>[8x]MIDLNIMKVANYINGEFKEPSTGAFQVKTSPVDGSKIAEVPRSGREDAREAIDSAFEALKAWANIPAIRRAEYLYKMLEVFRQMKEDFMKILTVEGGGTYRKVWGEVVFTERLIQNAAELARHYQGRVLQSDSESTISVVFKRSKGVVGVITPWNYPLSISMKKIAHTLAVGNTVVYKPASDTPVTGWLIAQMVAKAGLPKGVFNLVIGPGPVVGEEIVTHKRVAHVTFTGESSTGREIAAKAAGTLKTVTLELGGSDPLIILDDVDVDYAARLAVFASLFHQGQICTSAKRIIVHKAVADKFIERYVHYVKMLRIDDPRKDEKVDLGPLINERQVALMKEFVDDAVSRGGRLLIGGRSWGNFFEPAIFVDVDRNFRIMREEVFGPVRPIVVVENDDQAVEVANDTDYGLSGAVLTNNVNRAFRIAEAVESGMFHINDVTFLEESHVPFGGIKASGVGREGGEWSFHETTYDRWVTVTLRTRRFPIPSALK

In the present work, we report the structural and functional characterization of the first thermostable archaeal dehydrogenase (AlDHPyr1147). The kinetic data showed that AlDHPyr1147 is strictly specific for NADP+ and is active with aliphatic aldehydes. According to gel filtration, AlDHPyr1147 is a tetramer. The AlDHPyr1147 subunit consists of three domains: the coenzyme-binding domain (residues 1–256, 443–470), the catalytic domain (residues 257–442), and the oligomerization domain (residues 122–144, 470–491).

On the omit-map calculated for the model of the ternary complex without substrate, there were strong positive densities at the same place in the active sites of all six monomers (A, B, C, D, G, and H). Therefore, we interpreted this density as the substrate isobutyraldehyde. The oxygen atom of the substrate forms hydrogen bonds with the O7N atom of the coenzyme and the OG1 atom of Thr230. The isobutyraldehyde molecule is located at the bottom of the substrate channel at a hydrogen-bond distance from the coenzyme. However, it would not be appropriate to consider this structure as a productive enzyme-substrate complex or an intermediate compound since the substrate molecule is located at a too large distance from the catalytic Cys287 (the distance between the substrate and SG of Cys287 is 5.74 Å). The structure of the active site in the ternary complex is similar to that in the Holo-3 model, and NADP+ is fully ordered in the “hydride transfer” conformation. This is the only crystal structure of AlDHPyr1147 in which the occupancy for the nicotinamide ring is 1.0. The Cys287 residue has only one (rather than two) conformation, in which the side chain is directed away from the coenzyme. The other active site residues have the same conformations as in the Holo-3 structure. It can be concluded that substrate binding leads to ordering of the nicotinamide ring and the active site in general. In the ternary complex of AlDHPyr1147, the SG atom of Cys287 in the active conformation is at a hydrogen-bond distance from the peptide nitrogen atom of Thr288, and apparently this hydrogen bond can lead to a decrease in pKa of Cys.>[2x]MGSEVYQSQKCELKYSKSQIEKAARKIRHGCEGAE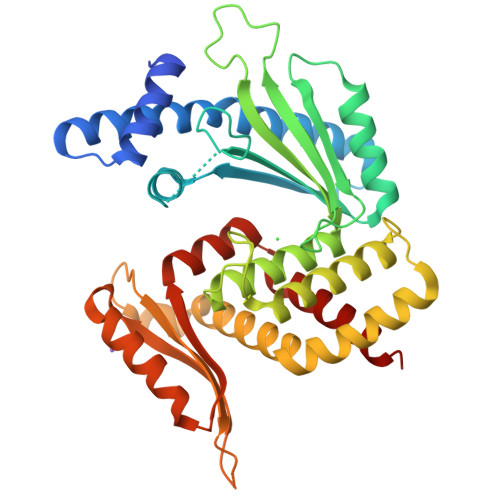REEAIKMIQNFRELHLYPLMLMKNHLDRAAKKVDKENKIIVARRLKRLSTIIDKLERPSLDGGATNNAIALTRMQDIGGCRAIVRNIEQLKKLKDRLVKSRSKHKILKEYDYLTPKPSGYSGIHLAYSCFDEENGNNPWSKTKIEVQLRTELQHAWATSLEIIDTLENIKLKTSNEGHPEWRRFFYLSGCLVAHDEGACILDDETIKNYQTELKTLEEALSVRSKLSTYTFAMKLTSDANLKKSLPKNHNGFFLVRMRNAITKNGKDTGKFLVSVKPFRKKESEQALQELNKDDADPEVLIAVLLATNNIKSLKKAYPNYFGSTNQFGRFLSRHIDTV>[4x]MRGSHHHHH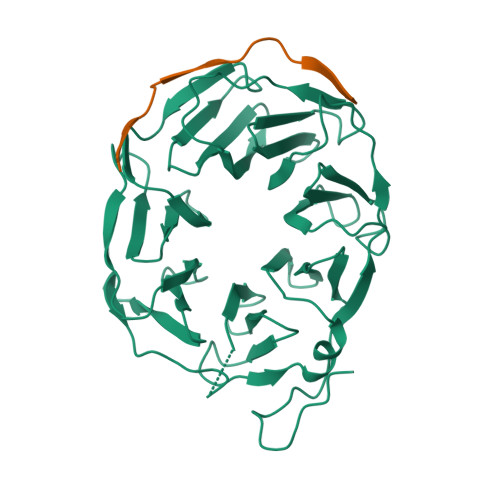HGLVPRGSIPALDYNPWEAIQLPTTATILDMSFIDRHHGWLVGVNATLMETRDGGQTWEPRTLVLDHSDYRFNSVSFQGNEGWIVGEPPIMLHTTDGGQSWSQIPLDPKLPGSPRLIKALGNGSAEMITNVGAIYRTKDSGKNWQALVQEAIGVMRNLNRSPSGEYVAVSSRGSFYSTWEPGQTAWEPHNRTTSRRLHNMGFTPDGRLWMIVNGGKIAFSDPDNSENWGELLSPLRRNSVGFLDLAYRTPNEVWLAGGAGALLCSQDGGQTWQQDVDVKKVPSNFYKILFFSPDQGFILGQKGILLRYVTDLTAAPA;>NAHNFPLDLASAESAPVA[2x]> GSPQDLTVSLIPVSGLKAGKNAPSAKIAKLVVNSTTLKEFGVRGISNNVVDSTGTAWRVAGKNTG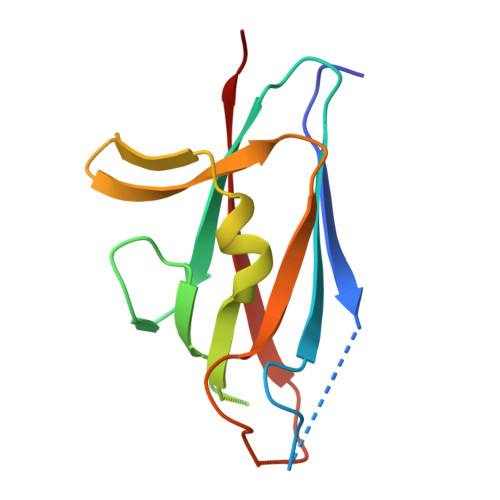KEIGVGLSSDSLRRSDSTEKWNGVNWMTFNSNDTLDIVLTGPAQNVTADTYPITLDVVGYQP> MSLLAKRIIACLDVKDGRVVKGTNFENLRDSGDPVELGKFYSEIGIDELVFLDITASVEKRKTMLELVEKVAEQIDIPFTVGGGIHDFETASELILRGADKVSINTAAVENPSLITQIAQTFGSQAVVVAIDAKRVDGEFMVFTYS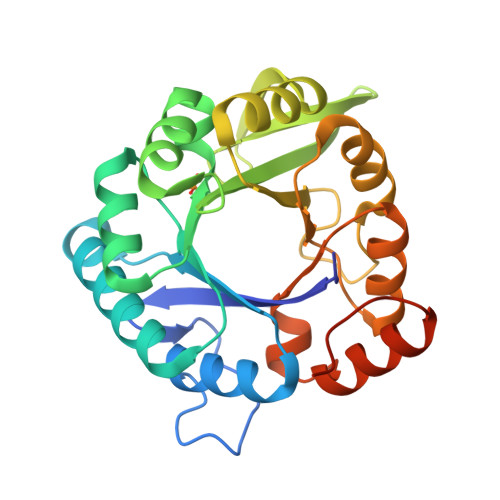GKKNTGILLRDWVVEVEKRGAGEILLTSIDRDGTKSGYDTEMIRFVRPLTTLPIIASGGAGKMEHFLEAFLAGADAALAASVFHFREIDVRELKEYLKKHGVNVRLEGLEGGSHHHHHH>MTARIALASLFVVAAVLAQPWQTTTQRWVLGVSIAAVIVLLAWWKGMFLTTRIGRALAMVRRNRAEDTVETDAHRATVVLRVDPAAPAQLPVVVGYLDRYGITCDKVRITHRDAGGTRRSWISLTVDAVDNLAALQARSARIPLQDTTEVVGRRLADHLREQGWTVTVVEGVDTPLPVSGKETWRGVADDAGVVAAYRVKVDDRLDEVLAEIGHLPAEETWTALEFTGSPAEPLLTVCAAVRTSDRPAAKAPLAGLTPARGRHRPALAALNPLSTERLDGTAVPL[2x];>MSENTVMPIVRVAVLAAGDDGGRLTEMALPSELPLREILPAVQRIVQPARENDGAADPAAAPNPVRLSLAPIGGAPFSLDATLDTVGVVDGDLLALQAVPSGPPAPRIVEDIADAAVIFSEARRRQWGPTHIARGAALALIGLILVGTGLSVAHRVITGDLLGQFIVSGIALATVIAALAVRNRSAVLATSLAVTALVPVAAAFALGVPGDFGAPNVLLAAAGVAAWSLISMAGSPDDRGIAVFTATAVTGVGVLLVAGAASLWVISSDVIGCALVLLGLIVTVQAAQLSAMWARFPLPVIPAPGDPTPAARPLSVLADLPRRVRVSQAHQTGVIAAGVLLGVAGSVALVSSANASPWAWYIVVAAAAGAALRARVWDSAACKAWLLGHSYLLAVALLVAFVIGDRYQAALWALAALAVLVLVWIVAALNPKIASPDTYSLPMRRMVGFLATGLDASLIPVMALLVGLFSLVLDR[4x];>FSSRTPVNENPDGVQYRRGFVTRHQVSGWRFVMRRIASGVALHDTRMLVDPLRTQSRAVLTGALILVTGLVGCFIFSLFRP[2x];>[2x]MSRLIFEHQRRLTPPTTRKGTITIEPPPQLPRVVPPSLLRRVLPFLIVILIVGMIVALFATGMRLISPTMLFFPFVLLLAATALYRGGDNKMRTEEVDAERADYLRYLSVVRDNVRAHAAEQRAALEWSHPEPEVLATIPGTRRQWERDPRDRDFLVLRAGRHDVPLDAALKVKDTADEIDLEPVAHSALRGLLDVQRTVRDAPTGLDVAKLARITVIGEADEARAAIRAWIAQAVTWH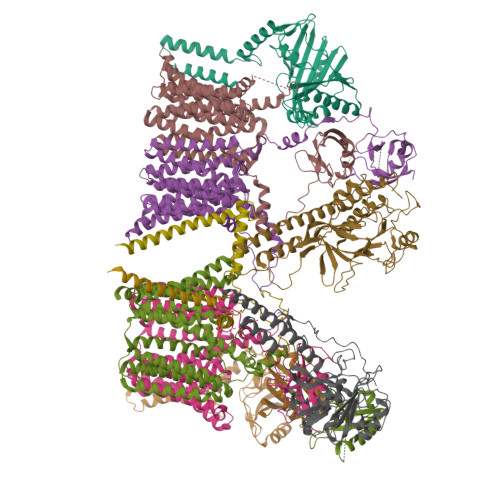DPTMLGVALAAPDLESGDWSWLKWLPHVDVPNEADGVGPARYLTTSTAELRERLAPALADRPLFPAESGAALKHLLVVLDDPDADPDDIARKPGLTGVTVIHRTTELPNREQYPDPERPILRVADGRIERWQVGGWQPCVDVADAMSAAEAAHIARRLSRWDSN> MYTAIPQSGSPFPGSVQDPGLHVWRVEKLKPVPVAQENQGVFFSGDSYLVLHNGPEEVSHLHLWIGQQSSRDEQGACAVLAVQLD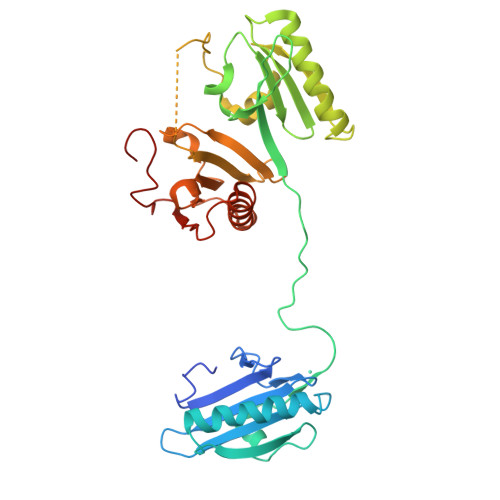DYLGGRPVQHREVQGNESDLFMSYFPRGLKYQEGGVESGFKHVVPNEVVVQRLYQVKGAKNIRATERALNWDSFNTGDCFILDLGQNIFAWCGGKSNILERNKARDLALAIRDSERQGKAQVEIVTDGEEPAEMIQVLGPKPALKEGNPEEDLTADKANAQAAALYKVSDATGQMNLTKVADSSPFALELLISDDCFVLDNGLCGKIYIWKGRKANEKERQAALQVAEGFISRMQYAPNTQVEILPQGRESPIFKQFFKDWK>[8x]MAHHHHHHSSGLEVLFQGPMTERLETRPQALLIKVPTEIVVKVVDDVDVAAPAVGQVGKFDDELYDEAGAQIGTSSGNFRIEYVRPTDGGLLTYYQEDITLSDGVIHAEGWAD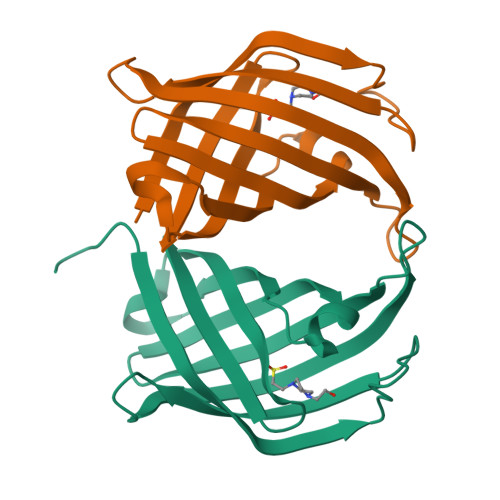FNDVRTSKWVFYPATGVSGRYLGLTGFRQWRMTGVRKSAEARILLGE>CCGGTACCGG[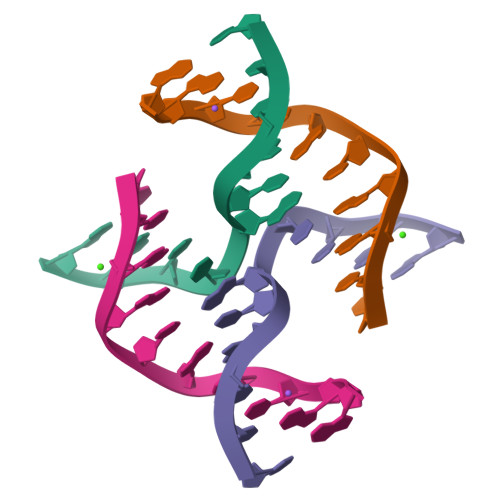2x]> MYTFSSKLKTFSIILMVLGLLGIGYGFLSAPKDIQEVEKILAADAHGAHGTAHGESAEASHKEAGHHEAAEASHEEHKGGEHAKVGAADEHTEHLNHVLHQLQNKPWSALYVACIFFLLLSMGVLAFYAIQQVAQAGWSPVLFRVMQGITAYLPAGSIIFFIILVLCGLHFNHIFVWLGEGVTDPKSPNYDAIIAGKSGYLNFPFWIVRAFIFLLGWNIYRHFSRKNCLAQDEANDDLYYKKNFKISAGFLVFFIVSESIMAWDWIMSFDPHWFSTLFAWYVFASFFVSGITSIALITIYLKSKGYLEYVNTSHIHDLAKFMFGISVFWTYLWFSQFMLIWYANIPEEVTYFVTRIQLYNLPFFGAVVMNFVFPLLILINTDFKRLNWVVVMAGIVILLGHYVDFFNMIMPGTVGDKWF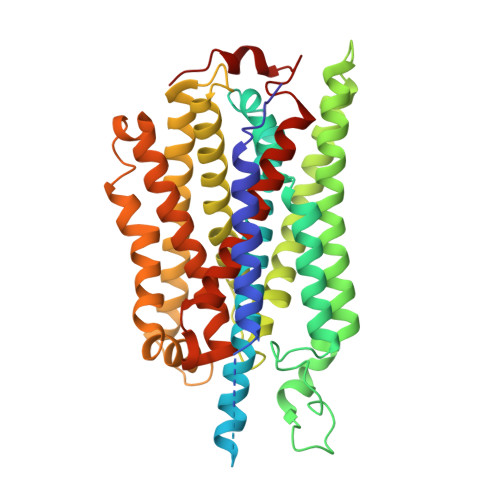IGVPEIASILFFLGLFIFVVFTALTKSPLLAKRNPFIEESKHFHY>MLLEGKTALVTGAGNGIGRTIALTYAAEGANVVVSDISDEWGRETLALIEGKGGKAVFQHADTAHPEDHDELIAAAKRAFGRLDIACNNAGISGEFTPTAETTDAQWQRVIGINLSGVFYGVRAQIRAMLETGGGAIVNISSIAGQIGIEGITPYTAAKHGVVGLTKTVAWEYGSKGIRINSVGPAFINTTLVQNVPLETRRQLEQMHALRRLGETEEVANLVAWL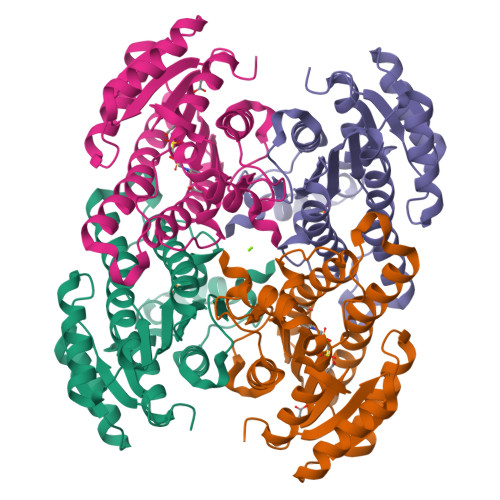SSDKASFVTGSYYAVDGGYLAR[2x]>[8x]GPLGSEEDVPENNGILISIKEVINAEFSRDGTIHSSELKGVLELRINDHDLSHSNLKLADSIDVRDKSFQFKTHPNIDKQS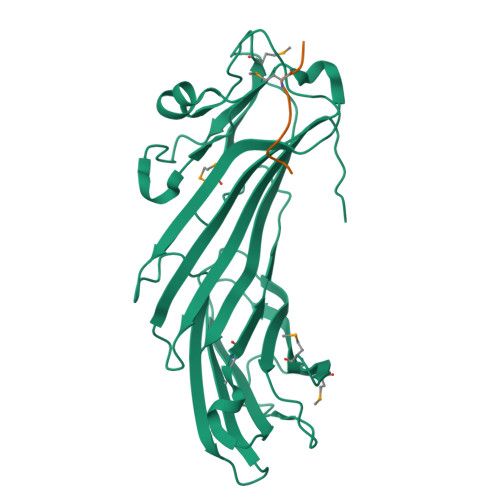FLSTKLISLRDKSKAFPANDQSLGVLRWRKVAPAEDDSLIPLTLTTAVSPSESQQGFDVIIEYESVLETELADVIFTIPVFPQEPVDINTESSTCSDAEVVNMDQEMGTSIKISKIAANDAGALAFTIEAPYEDALYPMTVSFQESTRDKLAKSFTGMAIQSVVMANDHDQELPYDVITSLKSDEYLVQ;>DDWNWEMED[8x]MGME1 (also known as DDK1) is a highly conserved, mitochondria-specific DNase. Human MGME1 (HsMGME1) protein is composed of 344 amino acids and belongs to the PD-(D/E)XK nuclease superfamily. However, in contrast to DNA2 (2–5) and many other mitochondrial DNases, MGME1 can cleave various types of DNA substrates with a preference for single-stranded DNAs (ssDNA). Structural analysis and comparison suggest that MGME1 follows a two-cation-assisted catalytic mechanism of substrate cleavage.

In addition to ssDNA2, we also successfully solved one structure of HsMGME1 in complex with DNA3 (5′-GGATCCTTCTTCTTCTTC-3′). Via the GGATCC located at the 5′-end, DNA3 can form a 6-bp duplex with a 12-nt overhang on the 3′-ends of both strands. The HsMGME1-DNA3 crystal belongs to the C2 space group and contains four HsMGME1 molecules per asymmetric unit. Three of the HsMGME1 molecules only recognize the 3′-overhang region, whereas the last one interacts with both duplex and overhang regions of DNA3. DNA duplexes normally adopt a B-form conformation, however, unlike the regular DNA duplexes, the DNA3 duplex is severely distorted. Though the flanking G1′ and A3′ still form Watson–Crick-like pairing with C6 and T4 of the complementary strand, G2′ does not form regular Watson-Crick pairing with C5. Phe173 is located in the middle of the α3 helix and its side chain stacks against the A3′-T4 pair of DNA3. Instead of stacking, the side chain of Phe173 directly points toward G2′ and C5, which leads to almost 90° rotation for both nucleotides. The weaker G1′–C6 pair and the irregular G2′–C5 pair all indicate that DNA3 is unwound to some extent. Trp152 is located at the single strand and duplex junction region of DNA3; its side chain is sandwiched by the sugar pucker of C6 on one side and by the side chains of Met156 and Phe165 on the other side.

>ESAALVAFSTSSYSCGRKKKVNPYEEVDQEKYSNLVQSVLSSRGVAQTPGSVEEDALLCGPVSKHKLPNQGEDRRVPQNWFPIFNPERSDKPNASDPSVPLKIPLQRNVIPSVTRVLQQTMTKQQVFLLERWKQRMILELGEDGFKEYTSNVFLQGKRFHEALESILSPQETLKERDENLLKSGYIESVQHILKDVSGVRALESAVQHETLNYIGLLDCVAEYQGKLCVIDWKTSEKPKPFIQSTFDNPLQVVAYMGAMNHDTNYSFQVQCGLIVVAYKDGSPAHPHFMDAELCSQYWTKWLLRLEEYTEKKKNQNIQKPEYSE[4x]> APSPEEKLHLITRNLQEVLGEEKLKEILKERELKIYWGTATTGKPHVAYFVPMSKIADFLKAGCEVTILFADLHAYLDNMKAPWELLELRVSYYENVIKAMLESIGVPLEKLKFIKGTDYQLSKEYTLDVYRLSSVVTQHDSKKAGAEVVKQVEHPLLSGLLYPGLQALDEEYLKVDAQFGGIDQRKIFTFAKKYLP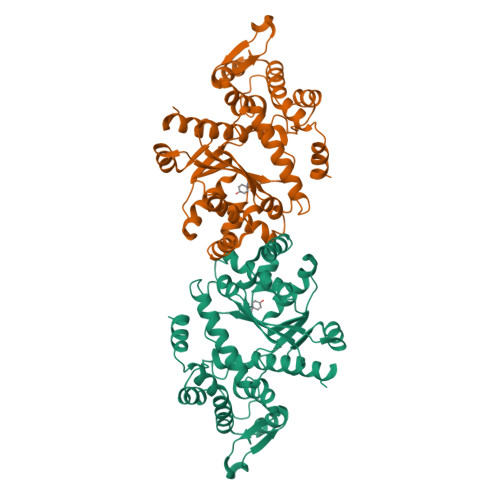ALGYSKRVHLMNPMVPGLTGSKMSSSEEESKIDLLDRKEDVKKKLKKAFCEPGNVENNGVLSFIKHVLFPLKSEFVILRDEKWGGNKTYTAYVDLEKDFAAEVVHPGDLKNSVEVALNKLLDPIREKFNTPALKKLASAAYP> GPMSEAADVERVYAAMEEAAGLLGVACARDKIYPLLSTFQDTLVEGGSVVVFSMASGRHSTELDFSISVPTSHGDPYATVVEKGLFPATGHPVDDLLADTQKHLPVSMFAIDGEVTGGFKKTYA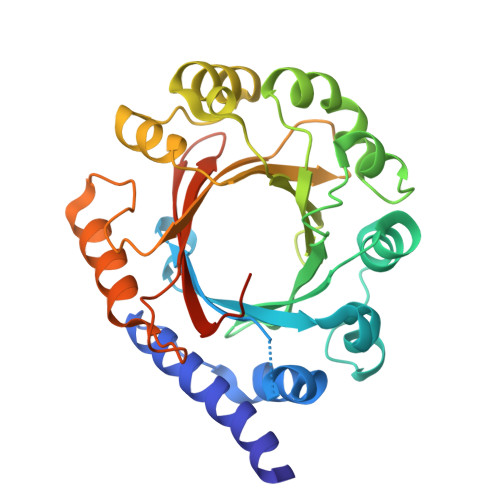FFPTDNMPGVAELSAIPSMPPAVAENAELFARYGLDKVQMTSMDYKKRQVNLYFSELSAQTLEAESVLALVRELGLHVPNELGLKFCKRSFSVYPTLNWETGKIDRLCFAVISNDPTLVPSSDEGDIEKFHNYATKAPYAYVGEKRTLVYGLTLSPKEEYYKLGAYYHITDVFRGLLKAFDSLED2-(6-AMINO-OCTAHYDRO-PURIN-9-YL)-5-HYDROXYMETHYL-TETRAHYDRO-FURAN-3,4-DIOL 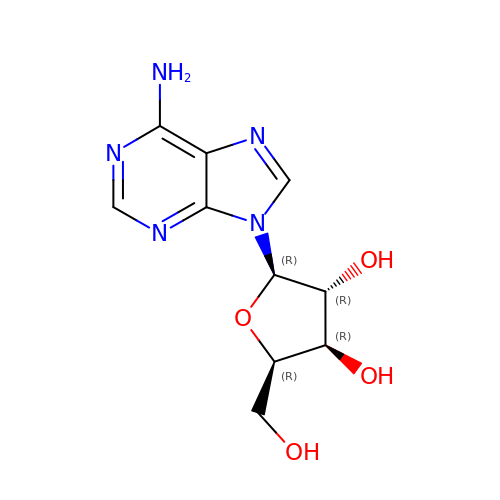| C10 H13 N5 O4 | OIRDTQYFTABQOQ-GAWUUDPSSA-N5-carbamimidamido-2-oxopentanoic 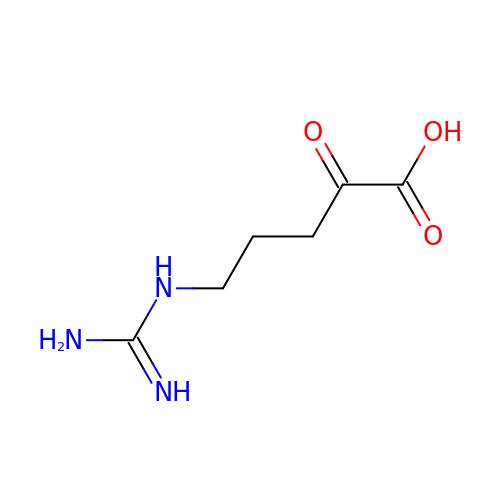acid | C6 H11 N3 O3 | ARBHXJXXVVHMET-UHFFFAOYSA-N>[2x]MKLQQLRYIVEVVNHNLNVSSTAEGLYTSQPGISKQVRMLEDELGIQIFARSGKHLTQVTPAGQEIIRIAREVLSKVDAIKSVAGEHTWPDKGSLYVATTHTQARYALPGVIKGFIERYPRVSLHMHQGSPTQIAEAVSKGNADFAIATEALHLYDDLVMLPCYHWNRSIVVTPEHPLATKGSVSIEELAQYPL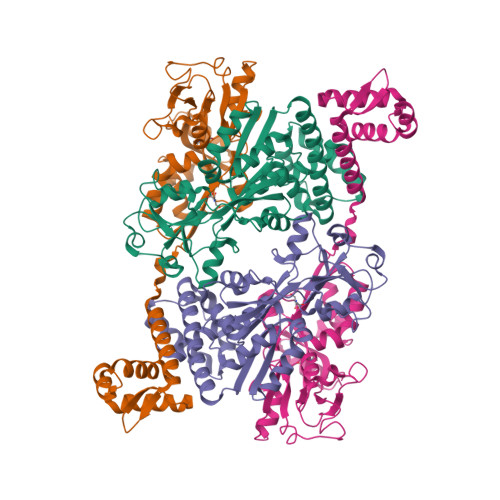VTYTFGFTGRSELDTAFNRAGLTPRIVFTATDADVIKTYVRLGLGVGVIASMAVDPVSDPDLVKLDANGIFSHSTTKIGFRRSTFLRSYMYDFIQRFAPHLTRDVVDTAVALRSNEDIEAMFKDIKLPEK> VVGGTDADEGEWPWQVSLHALGQGHICGASLISPNWLVSAAHCYIDDRGFRYSDPTQWTAFLGLHDQSQRSAPGVQERRLKRIISHPFFNDFTFDYDIALLELEKPAEYSSMVRPICLPDASHVFPAGKAIWVTGWGHTQYGGTGALILQKGEIRVIQQTTCENLLPQQI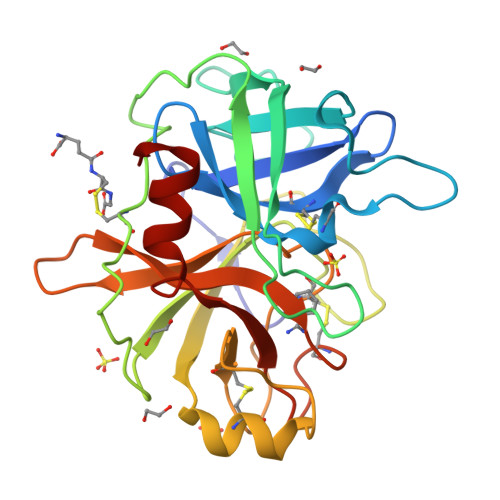TPRMMCVGFLSGGVDSCQGDSGGPLSSVEADGRIFQAGVVSWGDGCAQRNKPGVYTRLPLFRDWIKENTGV>MHHHHHHMAHFMDVHRGMHGITSDQLHQAHQADLAVEKDENVHFEQAWADPASGTIYCLSEGPSAEAVQRVHERAGHKADEIHEVPLSA[2x]

Here we showed that the 82-residue hypothetical protein SCO4226 is a nickel binding protein. The overall structure of SCO4226 adopts a ferredoxin-like fold with an α+β structure: five β-strands (β1-5) packing against two α-helices (α1-2). The N-terminal four β-strands β1-4 of one subunit form an antiparallel β-sheet, whereas the C-terminal β5 swaps to the corresponding β-sheet (β1′-4′) of the symmetric subunit, completing an extended antiparallel β-sheet of five strands. Each asymmetric unit contains a dimer of SCO4226, with a buried interface area of about 1100 Å2 on each subunit.

The two subunits of the dimer are almost identical, with an RMSD of 0.14 Å for apo-SCO4226, and 0.29 Å for Ni-SCO4226. Superposition of subunit A of the apo-SCO4226 structure against the ferredoxin-like fold domain of these structures revealed that the overall structures could be superimposed, except for the extension of β5 at the C-terminus of SCO4226. The hydrophobic core is formed by residues Met5, Trp41, Tyr50, Leu52, and Val78 from both subunits. One of the laterals is mainly composed of hydrogen bonds between Arg9-Nη1 and Glu74′-Oε2, Arg9-Nη2 and Glu74′-Oε1, Asp43-Oδ1 and Glu77′-Oα, Tyr50-Oη and His76′-Nδ1, Glu74-Oε2 and Arg9′-Nη1, Glu74-Oε1 and Arg9′-Nη2, His76-Nδ1 and Tyr50′-Oη, Glu77-Oα and Asp43′-Oδ1, whereas the other one consists of backbone hydrogen bonds (Ala40-Oα and Ala82′-Nα, Ala42-Oα and Leu80′-Nα, Ala42-Nα and Leu80′-Oα) from strands β2 and β5′, and vice versa (residues from the symmetric subunit were labeled with a prime).> GSRNQSPPQMMAQQGMHMQWTDQSFIEMMTPHHQDAID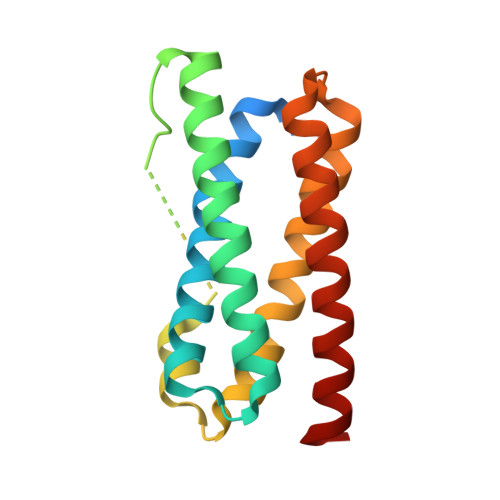MAEMALQKAEHPELKKLARNIIRDQEREIKEMKTWYQQWFKRPVPALSSQGMMGMHQGHGMMAMDLDALATAQNFDREFIRQMIPHHQMAVMMASNLKTNTERPEMDKLMDDIIRSQSAEIKQMKQWYQNWYGQ>DVNFDLSTATAKTYTKFIEDFRATLPFSHKVYDIPLLYSTISDSRRFILLNLTSYAYETISVAIDVTNVYVVAYRTRDVSYFFKESPPEAYNILFKGTRKITLPYTGNYENLQTAAHKIRENIDLGLPALSSAITT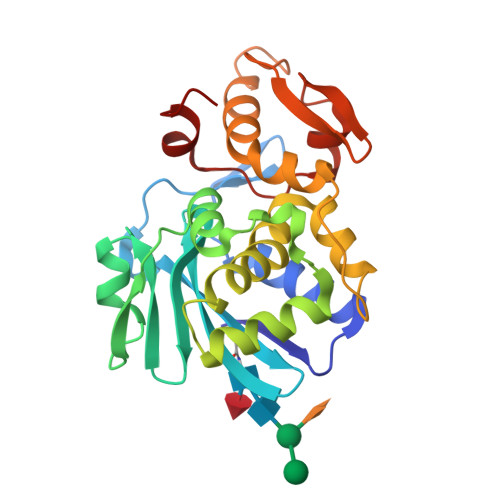LFYYNAQSAPSALLVLIQTTAEAARFKYIERHVAKYVATNFKPNLAIISLENQWSALSKQIFLAQNQGGKFRNPVDLIKPTGQRFQVTNVDSDVVKGNIKLLLNSRASTADEN[2x]>MALTTTGTEQHDLFSGTFWQNPHPAYAALRAEDPVRKLALPDGPVWLLTRYADVREAFVDPRLSKDWRHRLPEDQRADMPATPTPMMILMDPPDHTRLRKLVGRSFTVRRMNELEPRITEIADGLLAGLPTDGPVDLMREYAFQIPVQVICELLGLPAEDRDDFSAWSSVLVDDSPADDKNAAMGKLHGYLSDLLERKRTEPDDALLSSLLAVSDMDGDRLSQEELVAMAMLLLIAGHETTVNLIGNGVLALLTHPDQRKLLAEDPSLISSAVEEFLRFDSPVSQAPIRFTAEDVTYSGVTIP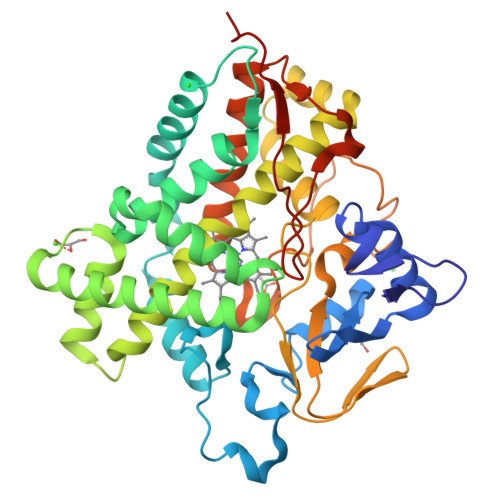AGEMVMLGLAAANRDADWMPEPDRLDITRDASGGVFFGHGIHFCLGAQLARLEGRVAIGRLFADRPELALAVGLDELVYRRSTLVRGLSRMPVTMGPRSALEHHHHHH[5x]N-(5,6-DIPHENYLFURO[2,3-D]PYRIMIDIN-4-YL)GLYCINE 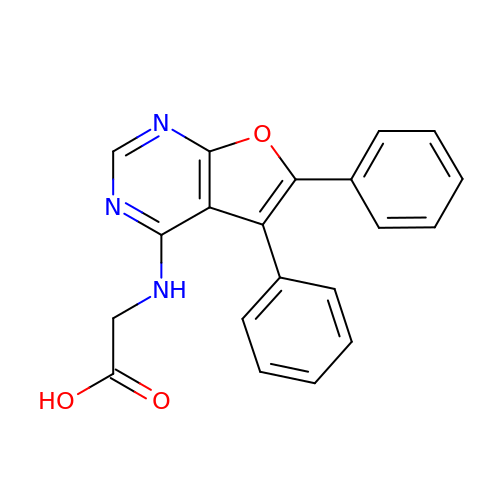| C20 H15 N3 O3 | VXTCEUDVOCLEJG-UHFFFAOYSA-N>[4x]SNAMERHQHLLSEYQQILTLSEQMLVLAT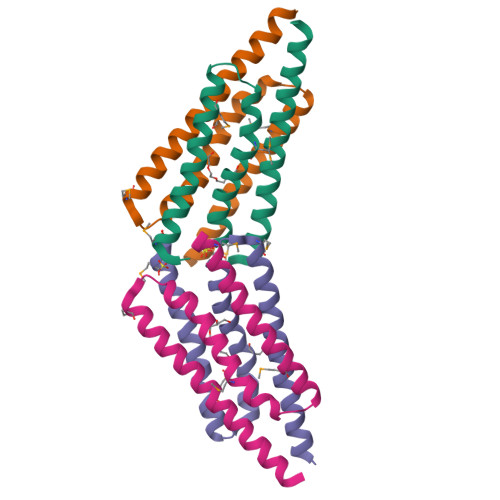EGNWDALVDLEMTYLKAVESTANITISSCSSLMLQDLLREKLRAILDNEIEIKRLLQLRLDRLSDLVGQSTKQQAVNNTYGQFPDHALLLGETQ> GMSAFDEFNEGFGLDVSDTPEELAFETESAIEEIESETSPGDQPKGSEPEEIRVWAEEKARKAVEEGREVTNWADWIMGWRTPNASEKKMEFMYWYTRTYLEEAKDIRPDIADALAR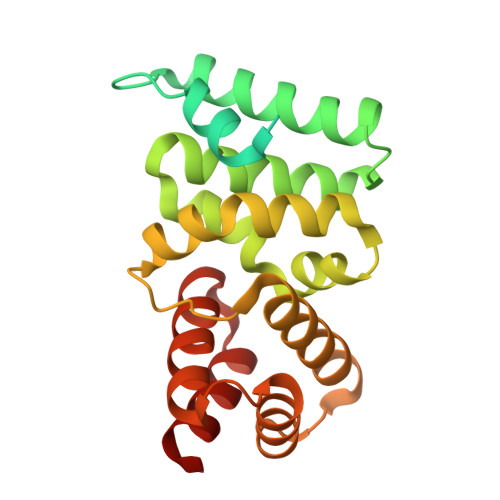GMAGLAFGRTDWVASMLDPQIMRHIYTDPEVARIYSETRDMLRRVSDYYISLTTMELGKVADIIAEAKAKGENPEVVAREIAEAVPRLSPKSLYFNLYYIGRSIGDNYVLEVARVLSKMRRR{3-[(5R,7S,8S)-8-azaniumyl-8-carboxy-2-azaspiro[4.4]nonan-2-ium-7-yl]propyl}(trihydroxy)borate(1-) 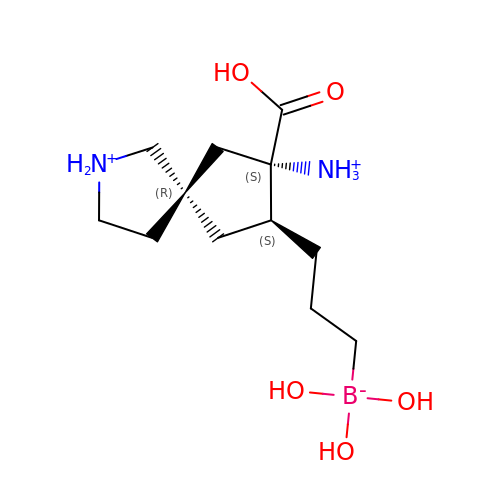| C12 H26 B N2 O5 | IOCRPFIKFQALKS-DLOVCJGASA-P>[5x]SSDGPGAAQEPTWLTDVPAAMEFIAATEVAVIGFFQDLEIPAVPILHSMVQKFPGVSFGISTDSEVLTHYNITGNTICLFRLVDNEQLNLEDEDIESIDATKLS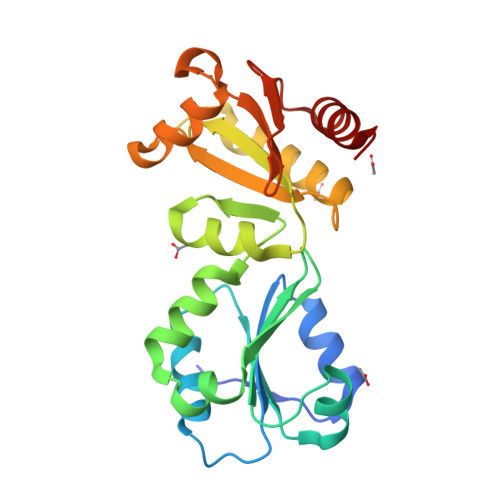RFIEINSLHMVTEYNPVTVIGLFNSVIQIHLLLIMNKASPEYEENMHRYQKAAKLFQGKILFILVDSGMKENGKVISFFKLKESQLPALAIYQTLDDEWDTLPTAEVSVEHVQNFCDGFLSGK>MAPSAYALDRSSVPSGKPRLMEGAESKARAGARKIHHLKIHGFDRVFGPGTHRWQRALWFAGVVFCFGISAHQIAMHVLDYLSEPVAVRIDFVAQNELRIPEITVCPRIFQQNTIFTDMVEKQGIDKMKFLDLIDRPEYDIMAVWNLSRIFSDNVSCSAHEGSSIISGSYVDPNMSQPHLVYTTSGQCINIPASRPLIYRGVNTFVRITDSQPRNLDEVRPEAIQIYFHEHHHAHLSRYLTGLRGYIVPIANPFAFSIRFTQINYANRTDSPCVDSEEYAACVEDFIEQRIYEKAQVQCRLPYMRPKLPLCSTPTDARKIFVATDDVIQNFEKESSCKRKCEE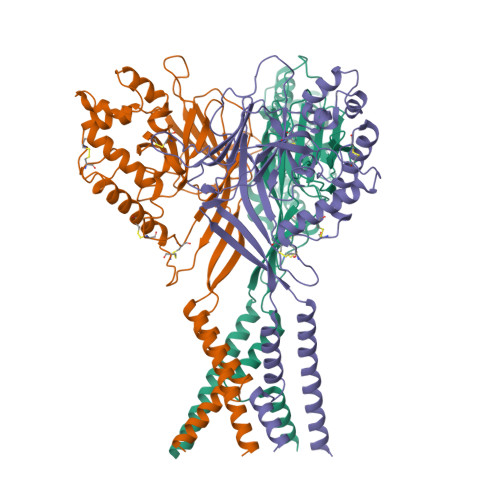NLYIVEFMHLFERSNISIDMSVYFAYNYIQVATEYLTYTLRGLLSDIGGVLGLFLGICILSVIEVFEVVIFSLQRVLCNEDKKQQNNE[3x]>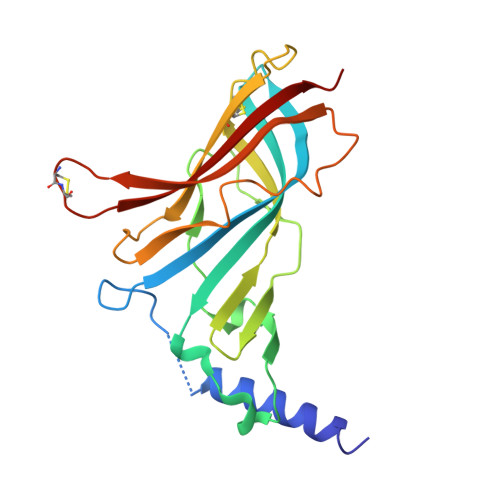 DDDDKLHSQANLMRLKSDLFNRSPMYPGPTKDDPLTVTLGFTLQDIVKADSSTNEVDLVYYEQQRWKLNSLMWDPNEYGNITDFRTSAADIWTPDITAYSSTRPVQVLSPQIAVVTHDGSVMFIPAQRLSFMCDPTGVDSEEGATCAVKFGSWVYSGFEIDLKTDTDQVDLSSYYASSKYEILSATQTRQVQHYSCCPEPYIDVNLVVKFRERR>[2x]MSGSHHHHHHSGSMSE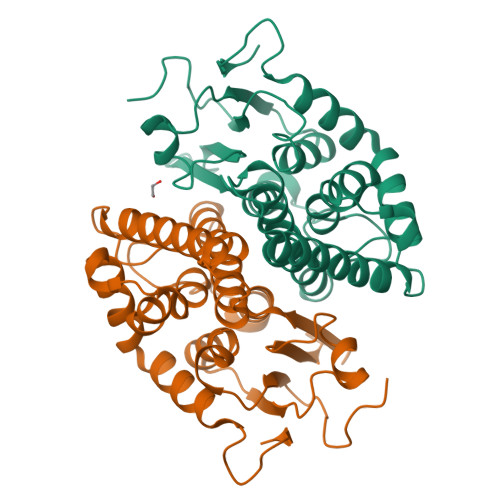RPSDLVVNRLVLFVVKGTATSTHNTVKPLILLEELGVPHDIYVVEKVSAPWFSEINPHKMVPAILDRSPDGRDTLRAWASTSTLMYIADAYDKDGTFGGRNVQERSEINNWLTLHTAALGPTAKYWLYFYKLHPEKLPKTIEKLRSNITVQYDILERRLNEPGQQYLALKDRPTIADIATLPFAMKSTAELFGLEFEKWPKLQEWSVRMGEREAVKRAWQRVAGFGHGEKEYGMLEA>[6x]ITYRDIVVKKEDGFTQIVLSTRSTEKNALNTEVIKEMVNALNSAAADDSKLVLFSAAGSVFCCGLDFGYFVRHLRNDRNTASLEMVDTIKNFVNTFIQFKKPIVVSVNGPAIGLGASILPLCD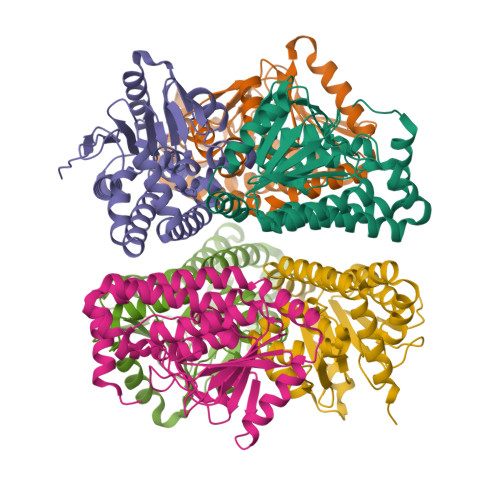LVWANEKAWFQTPYTTFGQSPDGCSSITFPKMMGKASANEMLIAGRKLTAREACAKGLVSQVFLTGTFTQEVMIQIKELASYNAIVLEECKALVRCNIKLELEQANERECEVLRKIWSSAQGIESMLKYVENKIDEF> MRKNIVAGNWKMNKTLQEGIALAKELNEALANEKPNCDVIICTPFIHLASVTPLVDAAKIGVGAENCADKASGAYTGEVSAEMVASTGAKYVILGHSERRAYYGETVAILEEKVKLALANGLTPIFCIGEVLEEREANKQNEVVAAQMESVFSLSAEDFSKIILAYEPVWAIGTGKTASPEQAQEIHAFIRSIVADKYGKEIADNTSILYGGSCKPSNAKELFS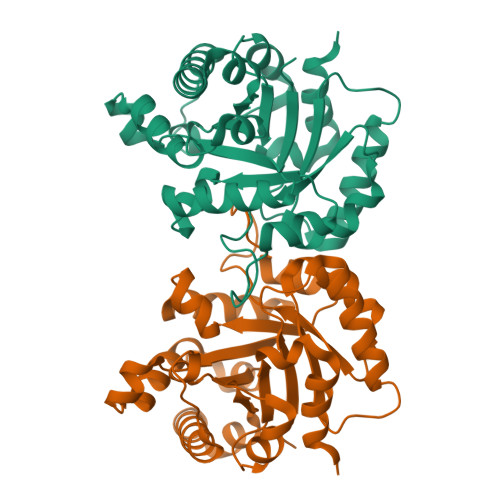NPDVDGGLIGGAALKVSDFKGIIDAFNA>MGHHHHHHHHHHSSGHIEGRHMMATNLRGVMAALLTPFDQQQALDKASLRRLVQFNIQQGIDGLYVGGSTGEAFVQSLSEREQVLEIVAEEAKGKIKLIAHVGCVSTAESQQLAASAKRYGFDAVSAVTPFYYPFSFEEHCDHYRAIIDSADGLPMVVYNIPALSGVKLTLDQINTLVTLPGVGALKQTSGDLYQMEQIRREHPDLVLYNGYDEIFASGLLAGADGGIGSTYNIMGW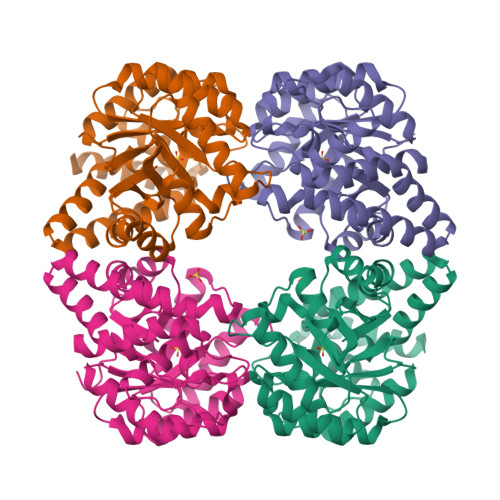RYQGIVKALKEGDIQTAQKLQTECNKVIDLLIKTGVFRGLKTVLHYMDVVSVPLCRKPFGPVDEKYLPELKALAQQLMQERG[4x]> MARRKCRNRFVKKNGQCNVEFTNMDDWPQRYIADMFTTCVDIRWRYMLLLFSLAFLVSWLLFGLIFWLIALIHGDLENPGGDDTFKPCVLQVNGFVA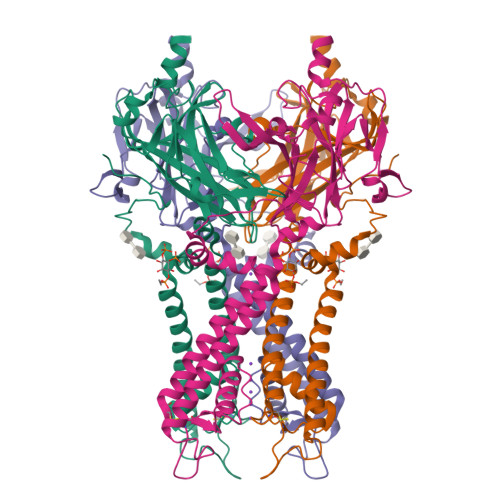AFLFSIETQTTIGYGFRCVTEECPLAVFMVVVQSIVGCIIDSFMIDAIMAKMARPKKRAQTLLFSHNAVVAMRDGKLCLMWRVGNLRKSHIVEAHVRAQLIKPRITEEGEYIPLDQIDIDVGFDKGLDRIFLVSPITILHEINEDSPLFGISRQDLETDDFEIVVILEGMVEATAMTTQARSSYLASEILWGHRFEPVLFEEKNQYKVDYSHFHKTYEVPSTPRCSAKDLVENKFLLSNSLEVLFQ> SGFEFHGYARSGVIMNDSGASTKSGAYITPAGETGGAI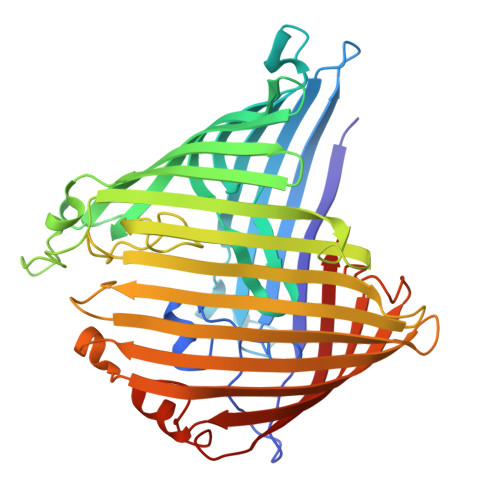GRLGNQADTYVEMNLEHKQTLDNGATTRFKVMVADGQTSYNDWTASTSDLNVRQAFVELGNLPTFAGPFKGSTLWAGKRFDRDNFDIHWIDSDVVFLAGTGGGIYDVKWNDGLRSNFSLYGRNFGDIDDSSNSVQNYILTMNHFAGPLQMMVSGLRAKDNDERKDSNGNLAKGDAANTGVHALLGLHNDSFYGLRDGSSKTALLYGHGLGAEVKGIGSDGALRPGADTWRIASYGTTPLSENWSVAPAMLAQRSKDRYADGDSYQWATFNLRLIQAINQNFALAYEGSYQYMDLKPEGYNDRQAVNGSFYKLTFAPTFKVGSIGDFFSRPEIRFYTSWMDWSKKLNNYASDDALGSDGFNSGGEWSFGVQMETWF1-[(5R,6R,8R,9R)-4-amino-9-{[tert-butyl(dimethyl)silyl]oxy}-6-({[tert-butyl(dimethyl)silyl]oxy}methyl)-2,2-dioxido-1,7-dioxa-2-thiaspiro[4.4]non-3-en-8-yl]-5-methylpyrimidine-2,4(1H,3H)-dione | C24 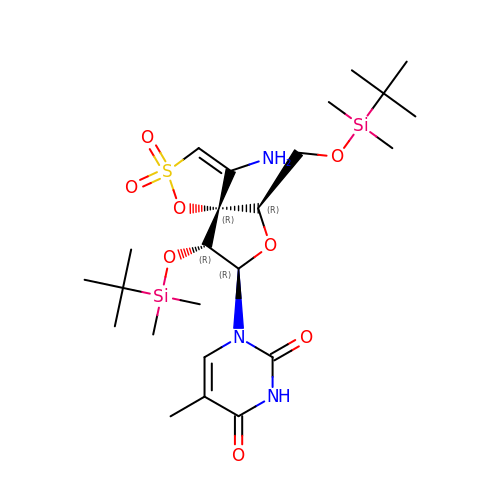H43 N3 O8 S Si2 | YMSLYTIPSGCZRM-DSPLJNTKSA-N> SLKRLAFSSLSHTLAPFPEGELDAHLSDADFTRVFTEEDDLDLVAQSLPLVLKVYEALHLQNPAHRGLSLAVGRLYIMYANAFVQTPAQYLPEDEFEAQNEAYSRARKLYLRGARYALSSLETAYPGFTREVFSGDE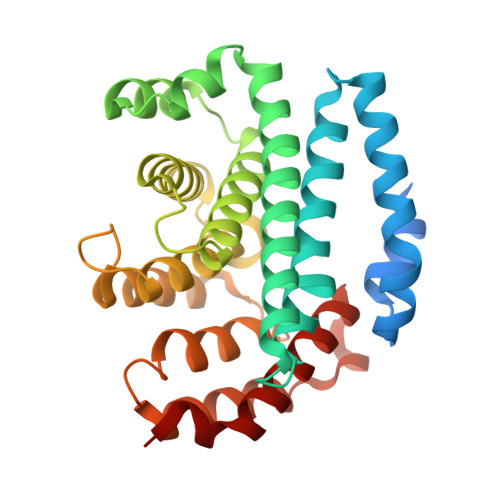QRLHKVLSRCTRVDVGTLYWVGTGYVAAFALTPLGSALPDTVHAAVMMLERACDLWPSYQEGAVWNVLTKFYAAAPESFGGGMEKAHTAFEHLTRYCSAHDPDHHITYADALCIPLNNRAGFDEALDRALAIDPESVPHNKLLVILSQKRARWLKAHVQDFFLD>LVATTSSKIYDNKNQLIADLGSER[2x];>[2x]SASNYPAYMDNYLKEVINQVEEETGYNLLTTGMDVYTNVDQEAQKHLWDIYNTDEYVAYPDDELQVASTIVDVSNGKVIAQLGARHQSSNVSFGINQAVETNRDWGSTMKPITDYAPALEYGVYDSTATIVHDEPYNYPGTNTPVYNWDRGYFGNITLQYALQQSRNVPAVETLNKVGLNRAKTFLNGLGIDYPSIHYSNAISSNTTESDKKYGASSEKMAAAYAAFANGGTYYKPMYIHKVVFSDGSEKEFSNVGTRAMKETTAYMMTDMMKTVLSYGTGQNAYLAWLPQAGKTGTSNYTDEEIENHIKTSQFVAPDELFAGYTRKYSMAVWTGYSNRLTPLVGNGLTVAAKVYRSMMTYLSEGSNPEDWNI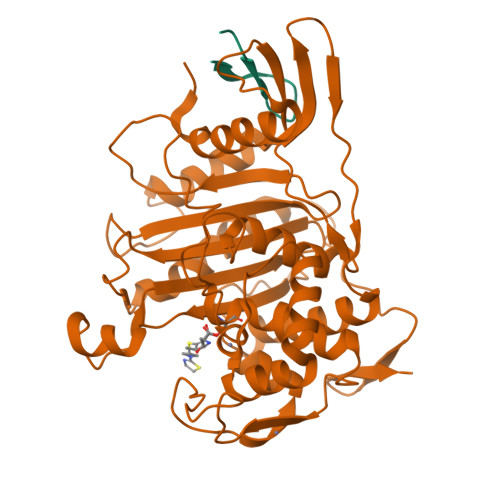PEGLYRNGEFVFKNGAR> MAELIPVENLDVVKAIVAEHREVPGCLMQILQETQLKYGYLPLELQGTIADELGIPLTEVYGVATFYSQFTLKPKGKYKIGICLGTACYVRGSQAIIDKVNSVLGTQVGDTTEDGKWSVDATRCVGACGLAPVMMINEEVFGRLTV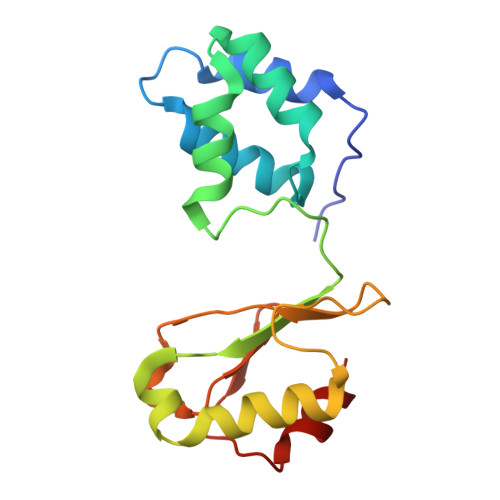DEIPGILEKY We investigated a TRPM2 chanzyme from choanoflagellates that integrates two seemingly incompatible functions into a single peptide: a channel module activated by ADP-ribose with high open probability and an enzyme module (NUDT9-H domain) consuming ADP-ribose at a remarkably slow rate. Using time-resolved cryogenic-electron microscopy, we captured a complete series of structural snapshots of gating and catalytic cycles, revealing the coupling mechanism between channel gating and enzymatic activity. The slow kinetics of the NUDT9-H enzyme module confers a self-regulatory mechanism: ADPR binding triggers NUDT9-H tetramerization, promoting channel opening, while subsequent hydrolysis reduces local ADPR, inducing channel closure. The structures of srTRPM2 exhibit a characteristic TRPM architecture, from top to bottom, a transmembrane domain (TMD) layer containing the ion-conducting pore, a signal transduction layer consisting of MHR3/4 domain and the C-terminal rib helix, and an ADPR-sensing layer consisting of the N-terminal MHR1/2 domain and the C-terminal NUDT9-H domain.

Before the onset of hydrolysis (substrate-bound state), both MHR1/2 and NUDT9-H domains are occupied by ADPR. Within NUDT9-H, the adenine group of ADPR is sandwiched by the indole group of W1264 and the phenyl group of F1372 via π–π stacking. The terminal ribose group of ADPR forms multiple hydrogen bonds with the side chains of D1330, D1426 and R1428. Three Mg2+ cofactors (Mg1, Mg2 and Mg3) are bound between the two phosphate groups of ADPR and two acidic residues on the Nudix helix, E1386 and E1390. The extensive interactions between ADPR and the NUDT9-H domain strategically anchor both termini of the ADPR molecule, exposing only its α-phosphate (Pα) to solvent and making it readily accessible for nucleophilic attack. Indeed, we observed a putative water molecule bridging Mg2 and Mg3, as previously found in the crystal structure of NUDT5. On activation by Mg2+ ions, the water molecule is deprotonated by the catalytic base D1460 located in a loop close to the Nudix helix, and is poised for nucleophilic attack on the phosphorus atom of Pα. Although both Ca2+ and Mg2+ activate the channel, the Mg2+-dependent ADPR hydrolysis of srTRPM2 is inhibited by Ca2+. This is because in the Mg2+-bound active site, the three Mg2+ cofactors are closely coordinated around the α-phosphate, likely inducing a favorable geometric distortion around the phosphorus atom for hydrolysis.

>[4x]MQRARPGELVEVIMFRPTGKARVSNLDESMAMEFTDLRTRAMSSAAMIRQSVAAKTLLIENEDGKGSTRMEVQDFMKRFHMHASEDDKTGSPSTAWGTLRFPTKEATAPYLRLSVNDDPEDALLFVKAMLAQKYGETYDRPSLILSVTGGARNFTLPPRLETAIAKGLRLAAQRTNAWVVTGGTNTGVMKLTGQIMEALSKTQSHFIPPTIGIATYGVIIGGDDMTRGEPPKIGLEYEMHKKDPPKTTPLDDNHNLFLLVDDGSTNKFGKEIKFRAAFENAAGQAFAAPVVTIVVQGGPGTLGTALQAVRQGTPIVVVDGSGLAADVLAYAYNFMHNPLTRFKSYTIDDLRQKVAQTFNPKSSQQLTNLLDSALECVQDPNLVVVYSLQESGIDEFDDCILKAIFSSQGKLGNKLKQAMYFDQLDVAKRALSEASKNGQHNEIAACINDNLMAAMMHNKPHFVELYLGFDAKIYELKPSEEVAKTNITALDELPSFALAIEELYKREAKKPHSHVQRLVSLSNTDVLGRHYRVSTQRGDGTTRRIGRDLANTRAYNVLRMDQIFARLVSKDFSVNRDFTIYDSKYDKVPGIQFRRTAQASHMLFLWAICLDRFRMARHFWLIGDQSIINALVASRILERLSTHRALQGPHLAEERAKMQHNAKKFEELAVGVLGECHGSDSHMASEMLHSKNDMFNKKNAINIAYDAKSLAFLSHPATQSVINADWYGHLKSVTSFWAVLFAFFFPFFVLPFINFSEDHAEQQVEAPRDFFTDAPRSSHSANSTTSGAHRLRRKFAKFYSAPYTRFISDLLSHFVLCVVTSYFVLDKLEDTISAIEWILLVWFVALLLEELRQMIFCDGIAEYISDTWNRLDLIMITLFFVGFFTHASDPSNQDSKVVSKGIHAFLVVVLWLRFMRYYALSKNLGPKLIMMMEMMKDVSTFVFLLLIFLIGYGVAAQSLLSPDEDFSSRTFIGVLFRPYFQIYGELFLDDLNSEANCLGDTPFTECSRETVRMVPFFLAVYILGSNVLLVNLLIAMFNDTYMKVQEAAEDLWRKQNYELCAEYKDRPFLPAPFILLAHVHMLFMRLLRLCGVHTQEHEKIQDDETKRKITTFEELNTDKFLRRWERERQEMLEARVKMTNDNVVQAMGMMDQLLEHMISFRFSLDQQATKIKQEIRDDGLPSTEPTGLVSRTPSQPINRLNSAVAVHGHTAEAAEWYVPPEEYPKSGGVKRYLIDASMVPLSIMCPSYDPVEYTHPSVAAQPVWADPADPRKIKFNVKDEVNGKVVDRTSCHPSGISIDSNTGRPINPWGRTGMTGRGLLGKWGVNQAADTVVTRWKRSPDGSILERDGKKVLEFVAIQRQDNKMWAIPGGFVDNGEDVALTSGREFMEEALGMGTSADLMSAESKDSLAALFSSGTIVARIYCEDPRNTDNAWVETTCVNFHDESGRHAARLKLQGGDDAEHARWMMVHGGLNLFASHRTLLQHVTSALNAYF The ESX-1 type VII secretion system is an important determinant of virulence in pathogenic mycobacteria, including Mycobacterium tuberculosis. This complicated molecular machine secretes folded proteins through the mycobacterial cell envelope to subvert the host immune response. All ESX gene clusters contain at least three or four ESX conserved components (Ecc), named EccB, EccC, and EccD, with EccE being present in all ESX systems with the exception of ESX-4. In this study we report the molecular structures of the periplasmic domain of EccB1 and the cytoplasmic domain of EccD1 from the ESX-1 cluster.

EccD1mt (Rv3877) is a 54 kDa protein containing an ~110 amino acid (aa) N-terminal ubiquitin-like domain followed by a 30 aa linker and 11 closely spaced transmembrane helices at its C-terminus. We grew crystals of the predicted cytoplasmic domain of EccD1 from M. tuberculosis (cyto-EccD1mt) which diffracted to 1.88 Å. We subsequently solved the 1.88 Å cyto-EccD1mt structure by molecular replacement using the EccD1mt segment of the MBP fusion protein. In both structures EccD1mt residues 20–109 adopt an identical ubiquitin-like fold characterized by a β grasp motif and an anti-parallel β sheet with strands in the order 2,1,5,3,4. Interestingly, the asymmetric unit of both crystal forms contains two EccD1 molecules and in both crystal forms the two EccD1 molecules are arranged as a head-to-tail homodimer stabilized by an extensive interface. The interface is formed by interlocking side chains from β strands 1 and 2 and the N-terminal α-helix of both EccD1 molecules and ~650 Å2 of each EccD1 molecule (13 % of the total surface) is buried in the interface as calculated with the PISA webserver. The interaction is stabilized by 4 hydrogen bonds and a cluster of buried hydrophobic residues including Met1, Val54, and Val58 resulting in a solvation energy of −13.9 kcal/mol and a Complex Significance Score of 1.0 calculated by the PISA server. Dimerization of cyto-EccD1mt creates a wide open-ended groove bordered on two sides by the α1/β3 loops. Notably, the dimerization interface brings acidic residues (Glu45, Asp49, Asp50, Glu57, Glu60, and Asp61) from both chains into this groove. The negatively charged groove of the EccD1 dimer indicates that it should associate with a positively charged partner(s).

>[2x]GAMATTRVTILTGRRMTDLVLPAAVPMETYIDDTVAVLSEVLEDTPADVLGGFDFTAQGVWAFARPGSPPLKLDQSLDDAGVVDGSLLTLVS hydroxy(2-{[(5S)-6-hydroxy-8-methoxy-4,5-dihydro-3H-imidazo[4,5,1-de]acridin-5-yl]amino}ethyl)dimethylammonium 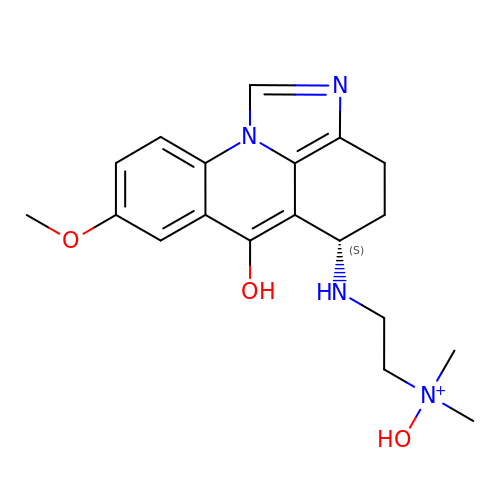| C19 H25 N4 O3 | VTPADFJSUDVABF-AWEZNQCLSA-O> PEAPYASLTEIEHLVQSVCKSYRETCQLRLEDLLRQRSNIFSREEVTGYQRKSMWEMWERCAHHLTEAIQYVVEFAKRLSGFMELCQNDQIVLLKAGAMEVVLVRMCRA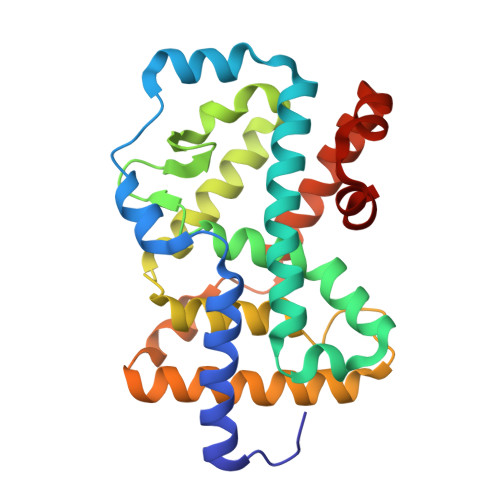YNADNRTVFFEGKYGGMELFRALGCSELISSIFDFSHSLSALHFSEDEIALYTALVLINAHRPGLQEKRKVEQLQYNLELAFHHHLCKTHRQSILAKLPPKGKLRSLCSQHVERLQIFQHLHPIVVQAAFPPLYKELFS Ciliary motility is regulated by the conserved nexin-dynein regulatory complex (N-DRC), which links adjacent doublet microtubules and regulates and coordinates the activity of outer doublet complexes. The N-DRC is a large 1.5-MDa, ~50-nm-long Y-shaped complex with two main regions: the base plate and linker regions. The N-DRC bridges neighboring DMTs and restricts sliding motions between DMTs. Here, using cryo-electron microscopy in conjunction with biochemical cross-linking and integrative modeling, we localize 12 DRC subunits in the N-DRC structure of Tetrahymena thermophila.

Here, we use integrated modeling and cryo-EM to model the entire N-DRC structure and some associated proteins from the ciliate Tetrahymena thermophila. In addition, we reveal that the N-DRC is associated with a network of coiled-coil proteins that most likely mediates N-DRC regulatory activity. We localized CFAP337 and CFAP57 and showed their interactions with the CCDC96/113 complex. We also find that the CCDC96/113 complex is in close contact with the DRC9/10 in the linker region. Our model implicates CCDC96 has crosstalk with the N-DRC. Therefore, the CCDC96/113 complex may function as a signal transfer bridge for the N-DRC that runs from radial spoke RS3 to DRC10 and vice versa. Our model revealed that the N-DRC is connected to an extensive network of coiled-coil proteins on the DMT that span the 96-nm repeating unit. Our structural model also shows that the N-DRC regulates ODAs and IDAs by interacting with a network of coiled-coil proteins. We hypothesized that the N-DRC conformation change during ciliary bending can be transmitted to the coiled-coil network by pulling force. N-DRC stretching can pull on the highly elastic coiled-coil protein network.

> MNPSQTQKGKIQIQVSRGSIDLLVRTMYEDINNIKLKNERFQKKKRAEDERRRRERYAEIQQEAIASGKKNAALEMKWAELKELDECEELNREMQDQQQTFQQIIEGKENLRKEFEEELKRKDDEYVKMLKEQSNDIKDMISKMRSQFYKIRDANMQELEDIERHFEQERSNLLNEFKAKIQATFKKHLDLEEQYVKEHAKTEEEQTKNIEDLRIKGAKHYAELKITMETEIQDLEKCFEDMKALYQLITEKLDYSLKVLQEKFHENNSMCDELKRKENNFKNRLKQLTKDYKQYDKKFKLENKNLTQEYKRIIRQFKELQKKFKHFEKADLDKYSEIQKMNEAEVKELKDKIIKCNITIHIQQLGMQWIPPQSEEEILAQQKLQLEQGGKAEEEEEREFEFCISEIKIGEICNIILEEADFLIDDKLREELEGSAEPEQIFQRLDCIKKCLYIDSEDEMNLFFRELITKCRVKSAEEIEEEARKQLLLLGLIKEAEENENPEGEEVQQQEGAQQKKKEEGNKKDDPKGKEGAKDSKENANPQGQNKSNQDERKKKKDGQDDHAGQGQGQYDSNQGGMGENQEEGENAEGQENLEGEIEKEIDLENTQINLNEVVKFLQNWQANKDKRKEKLEKESSKKAVKQETEREKKERIAREGKKYWEKLTQVLPERTFRIWNVNFFKFSFEKQILLNQINKLRFWTDLCPNIMNFFWTDKNQSKKPVNCITKMKNQRIFQINTYKLIMNLLSALQDSLIQIKDKDDFIQTKISTNLFTFHNFQILLQIFIVNQSFLFIRLCQSYSKKIILLIKNINQKLFNLSNFKNQFSF;> MALLGKTLKGRSTRPGGIPQKRNIKWRQLAKNQEEFDQLKQLAKMKREGLKARIKDEQKVVTFNKKKLITYWRKIMRIAKTEQLKNEIDIYSQNNQRELDSKEAFIQMLDKNLDEAEDQFQIALRNHLIHIENLMQLQEARMRGLAEEFNRDVNILETEFDLEREEMVKTHKTQLKELEDMIETVKEEDKKKTEEAQNEFSQFKEETKNKNLEETNVMKIILETKQTKYYTELEQMNSKFQSDTSNKVKDHQFYHAHNKNRKQEIDRYLRTISSKKAKIDLMKLKILQHCKEFNARNSALKKEKENISRNYHELKLKMQKFREEESRRLKELSNNSRNAVLKLREYCALGEKILKTAELCRRLETEKEKVLPFYESSVDEDQIPEQLKNEFEHLKKEDAEEYAYLNNFYKRYNKVLLDKLAIEKQKENLQRDNQLLKSLLKQYLDGISLNDDVLKNENNPLLVVNHKFNLGKMPVEKIENKTVIEGVFEVRNTSHQLQGQRAPPFQ;> MSNYISNYVQSTIVTKTVQNKDKKTGKNSVDPRVINEQLILDAVKQFNQENNKITTENIILQQLRQLQLSFKNILKIQHLQGLERLEKLQLDNNIIEKIENIDHLVNLKWLDLSFNCIKKIEGLDKLKELTDLSLFNNYIEKIEGLHNNTKLNVFSIGNNRLKSYEEITLYFGYKPRGEEGTNDRPEFKRLQVLNVSGNPFTKDKENEYKNHIICAIPNLKYLDYVFIDEGDRQLIRQDEQISNSYNFTTTDYYQQMQAQEQKEEMDRQTLKKKKDARMDILDNLKDEYLKIEDLQRVKIIKPNQINEEIEKYCGKINDHVVEMQAAVIQKHQLILQEMSKTEVSYKEQEALHEKETLQILKEFEHEKKVEFRNWEKEAANGDAKKEESRLKTLLQKTTSLKNKLMDIEIQLVEELEAIFTDYDTKKKETAWKDIEEIIVLGQKKIEEENVKFYSNLNVIKNKEEANYNSTQQQQLEEENNEEDDEKASLLENKEQLAQMIGNIKETLIDSHTKIILSAQMELQKDLAEYAKQQKNKMYERNRKNISQIIAQIDAYQTEINEKLKQGDDESDHEN;> MSKAAKAKKNVPVVSKLEADARKAAEGVNDNESEEFKKAMRKEARALVEQFNEEKKLLAFYQQERQKINYNWIIAKKELEDKKSELINKEREIQDLQENHFMTLNVYKQKIKHLLFQNQDQQSELKKDVEVTLKQLEDQHRIKSRELKTDVRSLKVTKKEQEISQQDYLFALKSEHDKQMTLMRQDYERQVNDIKRKYDLKMQNLTKEMEEARAAMIKQLEDNKNQKIAEIIKEHTQKYNDIKNYYSEITATNLDYRKTLKNEIKELQTKDEEYKKTLQQTEKGYKELNEPLQALGIEIIQLKKQDEEQEAIIKEKEELKQKIDNQERLFRKLEYEYEVKLQQFQYLERERNALYAKFNQTVFEIHQKSGLENLILEKKVTNLREDLEIKDLQIHQVLTAANIDPNSVGSINKSLEEVESLKNELISELQAQLKQIRKAHSHMVKAYEGKLSEFVIPVEELGFDPLVPTNTD;> MPPKKAKGKKKKEEEPDDEYKSMTGADLTQTLEKLKERVNEMRTNRNYIQMDRDMVENFYHNTLKEISEVKTKISNKETEAEEKESKHRIDVKVFLQKVKHLEYEQEKSNLNIEDDGKKAKEKEDAYFEDITKNMKQLKTQLKSEYLEKEKANIQQVQEEKKDHQSLLKIQQKKFDELINNLIIKYEERLAKLKEDLELKLKVEIHELEERKNLHINELMNNHEKAFAELKKYYNDITAENLNLIKAHKEKIAQIYANIQLNTKNVADNQAKNEQLKEPLAKHREIRNKLKEDLKQFAKHKMSLQNLKSKAITLKDKITKLERDGKDLDEKYEKVVREKQELEKKFEDITQEVKKNADLNNNVLSNRLQILLKEYNNKEEELRTIIDNAGLDHNLHEQLKQRVQQSIEAKNTLIKNLKYSIHHATKAYNDAIRVYEAKLVEFGIPIEELGFQPLETITSSMPAGLVSS;> MLAKKLALARSQGKPDPFKKDEFPLLQHIAVEVVSQNYILYPDLKGVPENVRDTIISKITTDLDILTMAPNIDQESFWQRACKNRWEKSQKSINIEEHGRSWKVAYLERYMEEFLTNIQNADDPNKKQILQAELKAAASWIHTLNLQNINQNIDIDFICKYLPLLTSLTLTYGTKYSGMDYNKQSVGMKLSEAANLGEAIKNCYSLLSLNISANMIDDDLLRFIMAGVNMNISLIELNLSHNKIEDQGARRIAKFLMRNEILLYLNLGNNLIGYEGSRYLAQALKVNKNLQSLNLKLNNLGDKAGKKLFQDLMLNKTLLELDVSGNQFEFETALKLSDYVADSMCGLKVLNIANNDFNDSCYENLKTGFTKNYSLAKLDLRGNKFSKTQEEKEQELKDPFRMFNLSQTEKELTQIIIRHDLTAQKIQFFSESDLDKIKQLKELQGAKQEPEKVIQQDQNKE;> MGDKKGKKKGGGEEDESTLQLSRQYKKKCELNGINPSKLFKEKLDFAVEEDENIEKIHLWEELGPVGVRSIMDSLTEIPYLHTKSIRLWKVKAQDEGTRTICNYMEKSKTIEYLDLMDNQVGSLGCEFLGRVLHPQIEIPLLKLKLDHNEFGTEGLMQLAAGLCMNSVLEKLSLNYCAITAEGSKYIQQILSFVNTNLKKLKMKGNLLKNEGVHQLFRAFKVNKTLEKVDLSDNQFDTTLGDDQDPEANPNFFETNKDAIEHNKQIIENICEVLKAADTLLYYDFRFNNISKTDAKAIIDCLEANKNIYYMELSEHIPKDLIERKKGLMKKRKPKKKKKKKAKKK;> MDHNEGGYSHHQIEGQEGQQQQAPVGGGGEDIFQVLENITQVQNEKLKRCQEFKEQENIPRQYIENSPKEELVLEHVIQFKRQFQYQLYYEDKRDLFLYPKNECDVYKFICTTIRPTKLGFLELYDYQQCSKYLSEFVQYEELDPPNEFPLVIPSPTNVAVWQKGDCFDMSILLCSLLIGVGYDAYCVYGKAPREITTRNESLMECLFLEKGKYIEENDKKPKQTLEQNENALLKKPIAHSKWDQTQETKAREAEEEKRRIALTINDDEPDELLEDPYQGQRVHCWVLLRSGKRDVQQNIFIEPSTGRMYSPSTCPYECVDAVFNNLNFWINMKPECEVKNLNFEEMDSSLNWEYVMLDTLLFNKGNGNDEEGNENIDDPLNKQAQRDPEQEQLQDIAQLLDMPPPWPPKIYIDKEKFLMGTPLGEGTVYYNKVKVDNYAPYSQPDGLVQKITIFQDYKRLKVKEYRYFYKHRSDKLSIRRRYPFEFKTIEEYEPQKYENKTIPQALQQWRQVIQIDRHLRIIKYYHNRNHDGLIERVEQIGEKTMMFYQNRDDRVIYRSIRFDNKRAPSSQNNDKVFQDNHVGDVQITKMTQKFEKNPHYPANEQIQKMVIDLIKDKVIVYYHMNDGEITPIVKIYPRDSMHGFAKLNEPGGDNKIDDPLVQLENTKMVNLEKDCLNQLKQQEKIARDDEKTIREGEIRLEKTLYDKARDRFKESSKKNDDDLAKDAAASDYLYPYLEKRKLLGVSEINAQVAMEIKNEVMQKLKERLLSRAEIIQRRLEEQRQVLEQKEAQVAKRQEIDPKQEEEIRDINFKIDILEQRALRFESMALQKYEEMDNRLNKDARLAALHRK;>MYDPNTSQTEKQKQEEFLKLKIQEAFNLFVKDKKGIVDKREIPYIMRYLGQFPSEAQVRDAILPEIEEDEPSEFIKYSKFEPYMLKVLKEREYEPDDPEALLAAFKLLDQEGKGYIEIDMMKTFLEKQGIEFREQETKSFIEFATNKDPNATVIYYEDYISRLQAFTDKHIESVMKGYNNFQVKK[2x];> MNQIDAHKLTIILRDATERLTFLDTINRQDDLSSELAGYEISKLLKKQKNLENQYADLVQLRTSLTGIQNKKNLIETQTKIVDVAQNLKESTKKLCRLFKENPDLESDALKVKKDRIQFMAVIEQLIQMVQNNSLTKFQSMTTLELEDQDRLRKLIFREKELYQEIKKLQFDRNQENKEYDNEQKDTNLKIQNLKERLLYKKARAQLKNQYKEKEARAEEGTQQRMYEFEQKQLKEKINNLKQKTDTENMVHEQLRNFLIEKEDQIKQKSDEWAKKVETCREQLQEEIDRLTVEKEKKQEELRELRERDQKEQEEKDRRERQELEEADRKQQEELDQIRLDNAIKLIQIEYQEWKDAGGGKKKRKKGKKKKK;> MQNLSKMQSRLHPRPEGEGGGGGGRTKEKGKSLQETHKEMLKNIESTNIGKPTIVEAQRILKIIDNLSTNLTIFIYLDSELISKFLDVAKHSKLSKDLVSKLSQRCLDLLKSQAEIEAKFKPYASLLDQSNKEAEDVEEEKMIDAERLRMQLENNFKDLVRHLRNSPEDFEIIKSMKTNVNPDLNDLVHCIHCQKVIMLKKLSTASEEDENHKAQLRDLEEKIEELEKKKNKIQEDLTKLKEHRQKFSKEKKEELEKLKNEIAEVKAEKEKKASQLKNELDNRLKQLERDHLAKKDKLDKELQKLEDDFAKLKQDHANDETKLKTNKRQQQNSLADNIESYDALMKDQHQKKQEIEEELAKIIEEVDTLKQLFKEIDEEKQRERELEEEFRLKKEQWEIQERRKKEAARCILHFLMARKEKSKKKKKKKGKKKK;> MSNMMYNMKWQEAINDLMEQVTLEYLPLEQNEQQLGMKYKRDSSEWFHFWATLYIKYIDIYKKLEDCYDQLVHPQKRVLLKEMLENVIVRLCETKSQVVKYNTQYDATYKSDYPNLDELVMDLKLTPDCLDIPIPRYFREEDKKRLDERNQILDALLLEYTDTKEPQEEQYEDQNTLQADMDTAIRIIQRYERGRQGIERANLAKILKKEEEKKLERQKKLAEGTEIGEETEKDDAALVIKKYWRGYKSRKLVQDIREEELLFLGMKKVVEDPTLPESQYKQAQNKRQKMKYIQEEHEQEFNDEIENLKRLVKGNEGPDILDKMRAERREWIMRELEKNEFKEAPQDPSEFYNQQVMDPEQQAAEAAKAAEEAKKKGAAKKDDKKKKGKPSELDEFLENNKPTGPSPIVLKLQEQIEKHSGEWSKRDETNNFEQKHETELAKMLIKPVVEEQIKQQVDEMIAEELDIVRLRYDIKKKKQKKPPRPRNKGKNKKKFPGDSSNKGRDPKDILAGLVEKRVAKKLIPASLMDLKGEQNVLGKIQEIQADENLKKTEALTDAKLKKAQLEEPSTKMPDPSIAQIRQIIAEYIAFPLGSKYAKEKLDKMNYFFFMGPRGSGKTLAVRALAHECNAIVLDISPSNIDGQYTDKKQIDGMINSAFKVAKEFQPAIIYCEDFEYIFGQAKKKKSQVNPLFAKMKKPLMDFKKGKFFEPEDRVVFIGSTNRPWDCSQKEIKSFFDKKIYFPFPNYGTRMLLFKTFLEQKKVPLPDNFPINTIAHITEGWSAGSFKMAIDRVFTERRLQKINEEQIKLSEFIGPLSNVPFTSKEEFKEFKKFNQVVTGLQANYEAKKAPADDQKGDKNKKKK;> MATTTNILHDVVRDQSMVNYVSNRDRPLYFKRPLVPQMTDIPLHISRPPVDQQVDYQTMQMQQNATIVEAPTKDAFVQTDYRESETQTDPYTPKCFVRDGDHPEVMELKDYKYGKGLPASIEELEQIELNREKVWFENSLPPISDEASFNLRRKLMEEQELREWSKKENEIKKFQNEKLYLLQQALIEREKEVEDKSQERIEEIRQQKTEHKNRQIAKIQRKKIKIDRKMTKSRKMQGKETLKRDIIEDYANFASRVYAGITHEGLSLDKIANKYEVQPLALGNYEMLQALHEGIRPREFETRVNLKKEIKEIEKNYTRLENYHRGELKKAQDEINGVHEQSKAQQKQEGNNFSYRNFENKIRPATPTWKYDTDFNISPSLITEIQEYRGPNGVQLMQAADKREEAVLLLQRLLRGRTTQNIMYEGKKKRTALIEELLTVAQIENLEEDKAEEVLMQQHEEKVKNAVLESIQGEVIAETMDELSKELLRIKQERKIQQMVEIAEKDRRIREIEEAGKRQAEEILRDREDVLHNQLIRVHQGTVDTYLDWLMSNALEQSSARQATIMTNLRKAKFNLPLEDFERKYNNNQTLIKDLVHSFLIPNVQRSKLKKQIQLEEKRFSEAAKRSLQQTITRASNKHANVQN;>MDQGEFIQDDNDQDYDQQEGDDENNDYMEDPQQDNNYNQNGDNLDDQGQDDDGGQNNLQQPSVPPEDDEDDDDDFPEYANEQNKRLNEIIKKKRKLIKDISAKIEEKSDRTKVLQEHLKNVEQELLHTQALIDAKNKEIETEDHMKQIAERQSGRIQSELKILEKRSIEQQEKLNDVQNQIFRGNEKMDQYKLEMNWNQEELEQWALAARQKEEDNLTLEKYKRADEVKIKELNLAIEKLTAEVGRKQNELEKEITETQAAQIELDKTAEEFKRQHEERHKLFLQWQEVTEIISKRDLAIREEGENFARIKIEIKSNKDALEERKRILKEAKEENKRIQMANELMERQNIQQISDNKHIEEQLAEKKADVEILKNQVSAFASDLSSKKNRIAILSQELLAKKQRLNAAQKKYQAHQVKLKNEEIMAKQYENDRSYAEEKYRKNEKEKKELEKEIRTQKENLFKHTQELFKHREREANLYGEIQGNMAACRNLQSHITKLNQEFQRQQELLYNAEYQIQLMERRVARAKGERTLEEKKDLENEIMNAERELGGVTGQNKELIESLKNLDDEIRTVKKKLAYVEEENTKYSSLIEELILENDMTYQDLNKIIKQKEEVLVQHDTMKLEIKKINESLNGATEKVFNLENQIYQLEMSMQEREKEIEVHKDVLMTEHKAAEEERHKIAVELAERKNKVKNLKIKYESLVQKNKASNGEVESVHEHSQAYYVIKAAQEREELQRKGDELNAKILKNEKELKALDNTLNHLKNRNSNYRDKFLNKGVTTQHREEAEGLEEQCRAASQNLFKKRDELQKLQKEQEEDTRRYTEIKNKLERLYEQHQSLDQEISKYQKDIDQQGDKLQRAQNSLQRNYQLAVNKNQNFINPKNPHMIQVKLDNQNNLYKTLLQGLYSLQQDIPELSSVVDEILKEQRIQNNKAPSSIDINSKRSSQSGRSQRSQRSNISNQ[2x];>MSNQQGPEDNNLEDDMAYLPADHPLLAKLQIDLTKQLTDEHERVDQKLIEIDANLKKLEKTKEDIGVRLYSVQQQLAENQMNFEQAHENYNWVQKLRIEAEQKLKTESEVYDAKKKELEELRKKYLKAQDELSKLTRTLYQINEFNQQMKGQIINTKTNTYRAEENVVNLEAQKKKQDLLIDTMNEEIKRQTEQKTILTAQLISQKEETEQAKQILKEAHLEMQKIIASKKNLLERWQKSLMTMQRMDNALQAIKEALKGQQELNLQIGTELNGVNAEIRKETEIQESLEGKNKKFDYEKDYLQKKYNELQEEKSKLEAQINLLTQSLRQTETEAGRAEIDKRNIEDQMNLIETNIMKLHTETKKLWEDLVHQKSEHTTIEKTATNLNKQANQISIEIEDKSVELENLLNEIARVKIDQLNTLSQIEVLENKRREVIKEREEKEITVATYEVQIRQGHDLNEKKQHEVGRLNREHDKLSSVQSDMSRGPLEAKRNNLIRKTQELGKENDLMQREWIKKQTLLVTQNNRLNKIEEDVSQLKTKQTILEQKKLRLNNNYRIYEKDIREIQNALKNLRNEMNKLNDAIYRNKEKQQKLDNENFNIKSEFVEKLKELEKESVKLEVEIDRLKEEKADLLAEIVESERQILLWERKIQLEKEMQDALDPTVGQTEIQELKREIHRMELRLDDLRKKQEAIIAEMERAVYKRETIQLKYMNKDKTFSNSNSMSQKSSSISAASDNSAQITKKIAQLKTTLNQTTRNAEQMEKAIKNKKIELDDLNAQIEGNNDNLQKLESDCYNKNIELTKHKLERSTNILSISCMQNKAKKLEDLVAGKARLSVPEATLMTKYEELRDKNQEIKEALQKLCDDAPQYVEVLNYLIDLNVGDDDEDQEQ[2x];> MASEDGEMPSQFEGIDPEQLTESQMQQYMMEMQRQGLLDSNMEGGQYEEGYEEGQEGEGYGEEYGDQDYDGNQNEYDSQQDSQQQGHDQVNEMHQDRYDRRVNSEISGNYEADDETLRKIRRDLLDNINLERRHRDLQPVYIDLTTNNISQYYSEYLVNNEHNQDFYENAKVRYNNLGECELCHITAKFEPDADITKEYIYDYFMEIGYLFLESEEEKRIILNPANNHIGIGVFFDEIQIVVVLILSEKVLCIQKISQPEQNKIEIRGKMLDENFGIYAIRIMNVDDQKKDIKGVGPEFIEYTRSTQEWMASFELELYNQDRMAIEYYTRVSPDSIPYKKKQSKNEKLTYKHLQLRLRTPFQIYPDPKYAAEDEKERIRKEQEILAHEEQERKEREENDAKRLKQSRKDYGDGQYDDDEHGQDDFNSQSDISDKDKHHDSMHAEQEQNQQAAQQQQDTISNKEIRQELEMAITEAQRQHDEFMLQNHKLQEEIKLLKNKNDGFVDRSNETAMNEHKYLNTLAHVHQIRLDLKQTQTRYNQMSQELQKKLEQKQKKCNEIKYAFLELKREVAKKAANSRTDKPIPEQQINEWEKAELQKSKELQELRLQILRLRNAYVKNQKILKKKEELAEGLHLIDFEQLKIENQTLNEKIEERNEELHKLKKKNTTTIQILTHTREKLGFVQGENGELNSQNVRKDQELDDMRKQLTQQKKTKDKLRSVNLTLKQQTGIVNSEELGQDYRDLRTRVSKLEEEKKRLEQKLRSMHEAIKTANQISTQNMQSQNNSLKKPYQPY;>MDNTGKLEKQLVTLNDGLPKKPAKEIIEELKHHLYQDFQKFFSEEKKQQYQNNFALFDRDNDKYINLSELKELLTSVNITFPDDELEELYNEFCLTSPEADGINEDAVFIIVSKKIRDNDKDEQLTQAFKLVEKAVNDELAKTPNETKEQEGYIRVEQFKELLMTLGNRWSEEQANEFLKDINPKSDERINYLDVVKKLMKR[2x];>[2x]MSKKSGKGKGKNDGDELGAEKEQVLRTKVESLIQRLGHEQERADRAKAAENELRARLFDLDKDFKNEKDRLFSITSDMTRQYKQMQDELLNQVNDLNKTVIEKDEEIKKKDQQIQDMTKDYEYKLKKKDDEIQDLKRKIEEMSAEFAKMLKDTLDKMQERIEMVQWDSDTDPQMMKRLKDMTGLSNN;> MNQDKHPEITDEEQELITVEELSQKLELLYKDMEQIRRENLLFEAYLARNRKEIAKEDEVSEDKKGKGKKKDKNVDKKSLLLTNEEKFEIAQQEQDALKKQIDDGRIKSDQILETLRAILEETDMAITEIRKDAFDFQREILVGGENSRTGKIEAEKIIKFFEEKERQKDALIAKYSSKRTNLERQILKTNNQIQKKEEMGDDLKFIDFYQLQIENKKYVKEIDDKNKKLLALKISTNRISQTLKDEKQNLKQELDKGKEYASQMSERKKKISKIDAQIKSVKKVTSKLEKDRKIYDKQKEIFVQDNQDDVPQIMKYVQYKSKEQQLLYAIQNLERKIEIAELAYKKANRILQSSQQFQQK;> MAGLAQHIQLKYIFGMNNEIRNSLQFHDEDRIIYPAGYNVVLHDLNDKSQHYYQGTNEYRGISCLALSPLKRYLALGVKGQRDPAIIIFDTFTQKRRKNLGLNLGNLDRYNIKQWVSIAFPSQNQETKYIFSLSGAGGDVVLCWWWHEKGKCLGSIDLGAQNDIYEISFNHSDANSICVTGNNFFGIYAKIEGTYVREDNQQKQKPSVQNGENSSAAQLPQPTLNIQVSAGNNNQNPQPEIKLENGNLISNLPADIVEKNFVAHLWMQCESYLVVFVESGEIILCDSRGNFLQIMEQSPRYFIVSRSGMIKIVAAVAYSKGFYVACSESIVLQYHYTQDNDKNPFTCVNQFKLKQFVELKEIEIKSICMNKAEDKLLIGLDNNQIYEIKIKPYHPETVNNDSSEDREVTLINHLNHTGPINSMDICKRKPIIATCSTDKTIKIWDYEKKQIKISWAFNEEAFCLSLHPQGFCVAVGFLDKLRLMNLCIHNSQNTTKNKAYKEISPFKGCKEIKFSNGGQYFAAVNSTSSNHVIQVFKFFTGENPSQLVFKGHTGRVKCIAWSSDDSFLLSCGLDGMILAWKLDQDFQHQQTIVPRIVDIHNKGVNFSGLTLTVDNKTIVAVGNDRHIHQAVINEQQPVDKTDKKLLDINLSCLAFPSSNKLLFAGIQDDARSSGAIRCFIYPLTHGKFTDYQAHDERGVEKMKITNDDRYIITAGKDGCIMVFEIKDKDARGMKLKDGYAKYSEEELITRSDLDDLKSTRDGLIVQINEFSNQNAMIGLNSRDDRIRQLETQIENNSQKRKQMFEQLLKSKTMEEQKLIQEINEIKEQFEQEIQVMDTKYQKEVMSLVEEYENQKRLHEIENNKNNKKKTKLLQEHSQKLQIIDDQYQKLLEEQITQKERVEKQINHLQKEQQEVLMQISEEKETEIKNLNQKNSKDEQAITDQGLKAKSDISITKKKIMQQQQEAQDLKEQKQEYERQKEKLKIQNQELRDKIDGQKKIILERDRTIGEKEKIIYNLKKKAQDLEKFKFVLDHKIKELKRDIVPREDEITKMKQETNNMDQYLKELNAYNNYLGTVVDELYTTQETMKEDIKQQRQQISVQQVKISRFKDDVYSLAQHILDYDKLVDETERLFMKHVNDKEVKRQSVEGDIMMEYRSQKKNLEKLVNMFKKSLQKDNQIHKDDKIRIMKDNVDLIREINTLRKSIKDITKGQQSNIPDQKGQTQHMPLQTPQLSRKSISQPVLPPISKSAMFEGVTQQNEIQKSHTQINPELVEEKQKVLNSLQTDILELQKVYEALNYEKHNLTQA;> MSSDVKDSSHLEKQNSQEYSNSKQNGEIDIMEMLPQKKMYIIEKQFDQSGKGLKIDEFVRVMLTHLDFDKSDVQKEDQITLALIDLFKEIDVNGDGTMEWEEFSDHIISLGLLRNDRSFKNVIKNYFPSEHIKDNQKHETPIEKIVYFDKLKYLVVLEKDSTRFKVYNANTAELYYEVNAHKCAVLDAEYIPDQNLIATSSNDLTINFWDSSFFIPKQIVSVPEIQLCMRYAKWSTQSQPTYLYTGGSDSIIHIYDTKTLKEKGTIGGWNPFFKRDSQQYGHASPIGDILPINIQTTLVTAGLDANICLWDAATHLPKKELRGHEKGVYSLDWSDFSPMNQCLLSAGLDHEAFVWNTYVKEKIFLLRGHNHPLIGVKCLPGTPQVITADINGMVKVWDVRNFLCMQTINVPTDELNSFVVTSNQKKRIIFGARRLYYYEYDEPKDQMLTDEKMCLRVLYNSVLLCLITLHPDCIKVWDIRTGKLQSVYRELSTAELTVCVLDTRKRKLFVGDADGNIFTVNIKNGAKMKKFEKHNNRMITDLTHWTSKKPATIEIGGDDDDEDGTGDSRRVVSCSREETVFIHDEDSSDPSRSCRYKMKQHKSSVNSLSLKQDSELFASASDDGNIVITNLNSYRQETLPSTQYPFEKKKVIFLDPYNALVTSDSEGYVHFYCVNNGKARTRYLLTKKYETTSVVNNKVDKFPVTHLAFNSDNNMLLLSDELGNVTIWDLTIFLKKLDEIKDDNIQQQKTKQAQTPLKQTPNRASNGFFPTELDELKQINEKQISLSQMDNLEKYFQDKDIAFVHQLKGAHNDGITWIEVLKEYNMFATSSFDCCCHLWSFNDYKKMGSLILGHDIMNNNWQLRVDEEKRKVDAQYYMEKLKKKLNKDDQSDDEEKNSQKQDESMMSDKNFDQKNQKKPKKTEKGEKGEKAPEKPLPEKKKVLTAQEKMEQNKKLKNELKLEFDPALLNLNKNKKQVLSEKEQIEKASELLEKVKKFNDVIANKNKDRRNPLEIDYDDFLRAYQMDEQVDIYLDQNEEEEEDNNILYDLDDPKNQSIPAGAYTSKGAFKSKNIGRKNKI;> MFKNTFQSGFLSILYSIGSKPLQIWDKSIRNGHIKRITDQDILSSVLEIMGTNVSTNYITAPADPKETLGIKLPFLVMIIKNLKKYYTFEVQVLDDKNVRRRFRASNYQSTTRVKPFICTMPMRLDEGWNQIQFNLSDFTRRAYATNYIETLRVQIHANCRIRRIYFSDRLYSEEELPPEFKLFLPIQGQNKTNV;> MAQQIVQSLQDEGTQSLKLDFSMKYVLGYRSDFKNNIFQYTMNDQNRIIYPAGNTIVISNNENKQQFINCIPGTKGITCMTLSPSKRLLAWSEDCDSGIIVVFDLIKLDKLEKAKNQNYQEPSDKDKLDKQAEKDRRDRFEKEKREKIDKLQKEVKRIITTLDCKSRHYVALDFNKINEKRIVALSCAPDWQLIYFQLDKQKTVIINQVPLKVGDNMRYTHCFFHPKEEDFIVAIGTGAIKPYKLGADGQFKQKDPPFVKKESKDQAHSPNYLSYCILQDGYMVIGTDMGEILLFQPSCEFKTILASSPKNEQFAIQCIQPYSKGFLVGGKECTILFYEKDVDLKNPYKLCSKKIQFRDMKAMITSLLLTPNEEKLIVGVDSGQLLQVPFTSDSMQLNEENSKCEPLFMPFHSDKITGLDVCIRKSLVATCSVDKTVRIWNYSDNQLENSKEFEEEAYAVAFHPSGFHIIVAFTEKIRLMNIFENDLISFKELSVKNCREIQFSNGGHFFAITNVSMVQVFQFYTGENPSNLVFRGSGKVRTIFWEEDDQGFYTGSTDGLVIYWRVDDNGPQKTQIAQFNNLIITSITGLYNPDTTTQGLERILFVSGVSSSQENEGEKCVYKLVISCRQDKEGREITDNTLKKIYYVSQPEQKIFTGTNVSQIAISHSKKLFFFATEDRPGAIRITKYPFTNEIMEIQSHFGPITRMRISFKDNYIFTAGEDGALIIYENKEKEYQVKIENESVEAAAEEFLIPRDQYNDQKREIEKLKRQLNEERMKQEQQIKEKMKDRDDKINQLENQQKDSDNRDLNKYQLLEREKNEMIESYEEKKRMMKLQHENNKRTIENEYKKKIALEMSRNEELAREKEKEEKRFQSEIQQYQEEHLRQMEEKRRHYEEQLAIEKQLYNDLHLKREELAYKFDQKRNKLEMEAEELIDQLKEENESKMQVLFKNLEKAEIKKMDRRNDYDTEAQKLEEQKSKLKGTMEDITSIQETNKMLQKEKESHAKEIDEREKTIRDKGRRIYELKKKTQELEKFKFVLDYKIKELKRDIGPKEEEIAKMKEQIANMNSEILHFKRTNANLKLIVTDLRLRQEGMKKEIEDQSKVIQQNNQYIKAFEQDMSDCHQHIADYKKLKQKVLNLYNQYVQGDDSKKKRLENNDQQKEIMKERAHLETSVNNLKIKHDKNQSVHKSDTTIIMKHNTFLIFEINHLKREKKKILEDKAKMLMQATQKKKQDGTSRVDIDSLEKEIQKNEDEKRKLKEDIEKLRQYNDQIKNQLRQQIQNQQDDDEDN> QG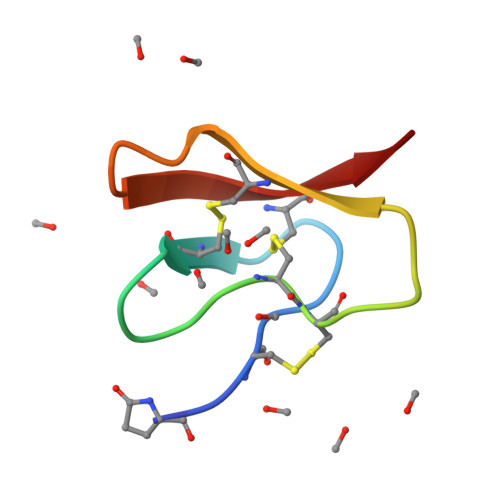CAFEGESCNVQFYPCCPGLGLTCIPGNPDGTCYYL>MTSSVLAALLSVSIMLVQLRAEANIGTGDNVLHRAALCGIIELAGKRAKLETALPNFQNELNSILELNMTAAEPTWLDQFRDKDDRSKPRDLTKQPLPKDTNWADHWTAWAKAALPLLNDETHQAKLKEYKLAGLQPEKLERARNTIRRLTAEAVAKAQDPTVAESTADLTTEEDLQKQINQAVYSKDTEPDDDFNGYTAFEGKASTNRQTICGSAVAGSKATNAMDALFCVCADDRTNGADAGKACVAGTAPGTGWNPGVTATPTGTMLQKVRKLCNTHGKTTLSAAAIEGRLTAVGNLLTRGSATSILGSFLATDCSGDQGSGMCVAYTEVTDAKGTPTKDIPWMQKLDSVRIKLQKHERAVEKLGKPQHDLKTILTLAKDPAYLQLASVGTRHLETTKQRVSNEQGK[18x]

Long-term immune evasion by the African trypanosome is achieved through repetitive cycles of surface protein replacement with antigenically distinct versions of the dense Variant Surface Glycoprotein (VSG) coat. The mature VSG proteins are attached to the cell surface by a GPI-anchor, and consist of two main regions: (1) a large, N-terminal domain (NTD) of roughly 300–400 amino acids that is most distal to the membrane and (2) a smaller, membrane-proximal C-terminal domain (CTD) spanning 80–120 amino acids beneath the NTD that harbors the GPI-anchor. Therefore, at the heart of antigenic variation in the African trypanosome are the NTDs of the VSGs. These large subdomains are elongated folds centered on a three-helix bundle scaffold.

An additional crystal form of VSG11 shows non-crystallographic trimerization in the asymmetric unit, while another form also raises the possibility of an inherent flexibility that could be present in the VSG proteins. In a second crystal form (VSG11N2C-18mer, determined to 2.6 Å resolution), the asymmetric unit contains six trimers of the same arrangement as observed previously for all class B VSGs, for a total of 18 independent molecules (hence “18mer”). In addition to helping establish that this specific trimeric arrangement is the preferred oligomerization of this class (at least at higher concentrations), the independent monomers in this asymmetric unit display a range of alternative conformations, particularly in the bottom lobe of the protein and even in some limited regions of the three-helix bundle. An overall structural alignment of the monomers to themselves gives an average RMSD of 1.33 Å (RaptorX), a somewhat high value for aligning a protein to itself. Examination of the set of alignments from the monomers of the 18mer show that it appears that the divergence primarily occurs in the lower lobe. Finally, when the different monomers of the 18mer are compared with the other crystal forms described, a wide variety of conformational changes is seen, although these changes are limited to the bottom lobe and lower regions of the bundle. Due to the high flexibility of the bottom lobes in the 18mer crystals, not all amino acids in some monomers of the bottom lobe could be modeled.>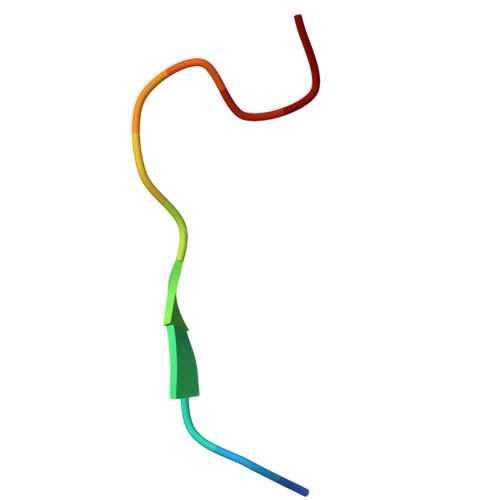 GLPVMNTPGSNQ>[4x]MASTKTPRPYSEIPSPGDNGWLNLYHFWREKGSQRIHFRHIENFQKYGPIYREKLGNLESVYIIHPEDVAHLFKFEGSYPERYDIPPWLAYHRYYQKPIGVLFKKSGTWKKDRVVLNTEVMAPEAIKNFIPLLNPVSQDFVSLLHKRIKQQGSGKFVGDIKEDLFHFAFESITNVMFGERLGMLEETVNPEAQKFIDAVYKMFHTSVPLLNVPPEL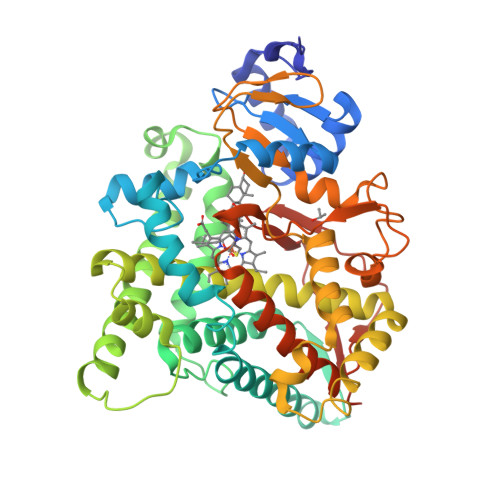YRLFRTKTWRDHVAAWDTIFNKAEKYTEIFYQDLRRKTEFRNYPGILYCLLKSEKMLLEDVKANITEMLAGGVNTTSMTLQWHLYEMARSLNVQEMLREEVLNARRQAEGDISKMLQMVPLLKASIKETLRLHPISVTLQRYPESDLVLQDYLIPAKTLVQVAIYAMGRDPAFFSSPDKFDPTRWLSKDKDLIHFRNLGFGWGVRQCVGRRIAELEMTLFLIHILENFKVEMQHIGDVDTIFNLILTPDKPIFLVFRPFNQDPPQAHHHH> GSHMAFIERPEDFLKDKENAIQWEKKEAERVEKNLDTLEKEALELYKKDSEQISNYSQTRQYFYDYQIESNPREKEYKNLRNAISKNKIDKPINVYYFESPEKFAFNKEIRTENQNEISLEKFNELKETIQDKLFKQDGFKDVSLYEPGNGDEKPTPLLIHLKLPKNTGMLPYINSNDVKTLIEQDYSIKIDKIVRIVIEGKQYIKAEASIVNSLDFKDDVSKGDLWGKENYSDWSNKLTPNELADVNDYMRGGYTAINNYLISNGPLNNPNPELDSKVNNIENALKLTPIPSNLIVYRRSGPQEFGLTLTSPEYDFNKIENIDAFKEKWEGKVITY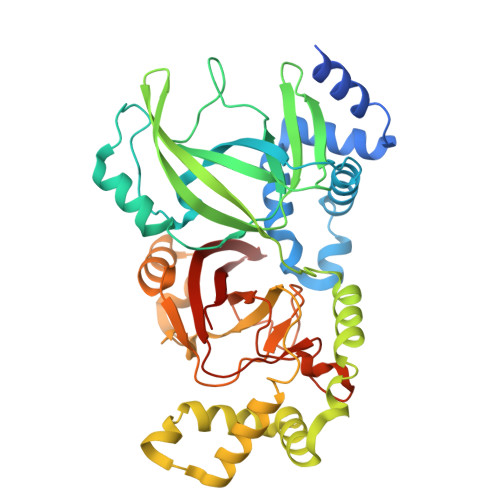PNFISTSIGSVNMSAFAKRKIILRINIPKDSPGAYLSAIPGYAGEYEVLLNHGSKFKINKVDSYKDGTVTKLILDATLIN>[4x]MHHHHHHENLYFQGAGAGAGAGAMATARELHDVIVETRYGAVRGRSDGTVCVWKGVPFARPPVGPLRFRPPEPPEPWSGVRDATRFGPASVQPEDRLISNLTGGATLPQDEDCLYLNIWSPSPDGRRPVMVWIHGGAYLTGAGSIPWYDGTALAREGDVVVVTLNYRLGALGFLYLEDAFGPEFTGSGNLGILDQIAALRWVRENIAAFGGDPDRVTIFGESAGAGSVGVLLAAPAARGLFHRAILQSGSGALGVRTAASAARVAARVLQHAGVEPGDREALRSLPARAWANAVAALGPGLPLGPVVDGTVLPEHPMAALARGAA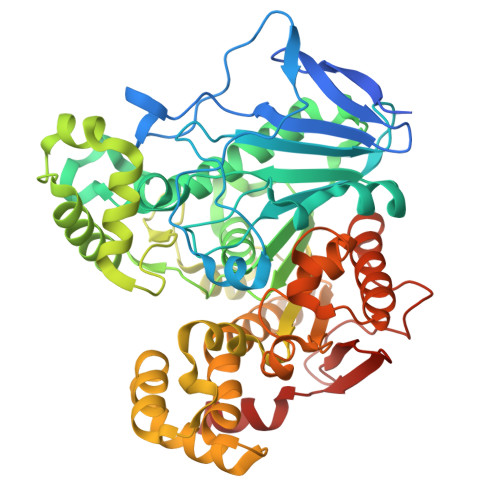RDVAVLVGVNKDEYNLFALQDPAWLGDDEAALRQRVEAVVGPAAGRLIEFYRSRGEGSLGRRLLPLMSYAVFVRGMLATADAQARVGAPVWAYRFDFETPVLGGVLGACHALEIPFVFNTLDRAGADRFTGTAPERYAVAQAMHRAWIAFAREGNPQHDGLPEWPRYDLEERAVMVFAVEPRVERDPWRAEREVWAAAGVGA> MGIQGLAKLIADVAPSAIRENDIKSYFGRKVAIDASMSIYQFLIAVRQGGDVLQNEEGETTSHLMGMFYRTIRMMENGIKPVYVFDGKPPQLKSGELAKRSERRAEAEKQLQQAQAAGAE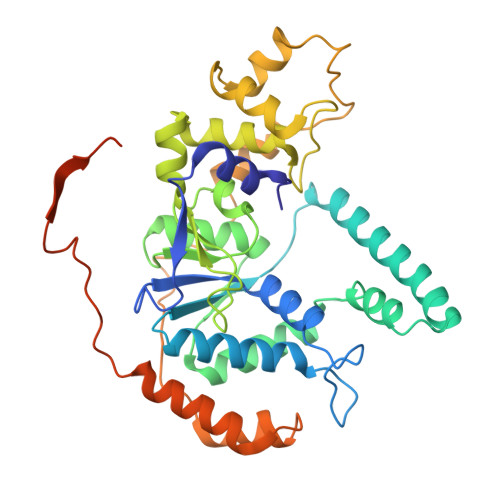QEVEKFTKRLVKVTKQHNDECKHLLSLMGIPYLDAPSEAEASCAALVKAGKVYAAATEDMDCLTFGSPVLMRHLTASEAKKLPIQEFHLSRILQELGLNQEQFVDLCILLGSDYCESIRGIGPKRAVDLIQKHKSIEEIVRRLDPNKYPVPENWLHKEAHQLFLEPEVLDPESVELKWSEPNEEELIKFMCGEKQFSEERIRSGVKRLSKSRQGSTQGRLDDFFKVTGSLSSAKRKEPEPKGSTKKKAKTGAAGKFKRGK> MSQLVFIVFQDNDDSRYLAEAVMED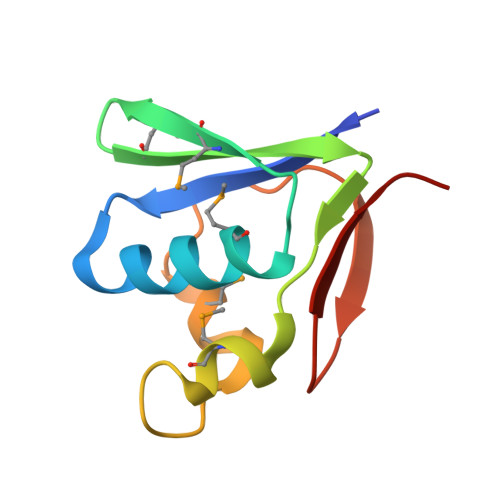NPDAEMQHQPAMIRIQAEKRLVINRETMEEKLGRDWDVQEMLINVISIAGNVDEDDDHFILEWN> MAVSV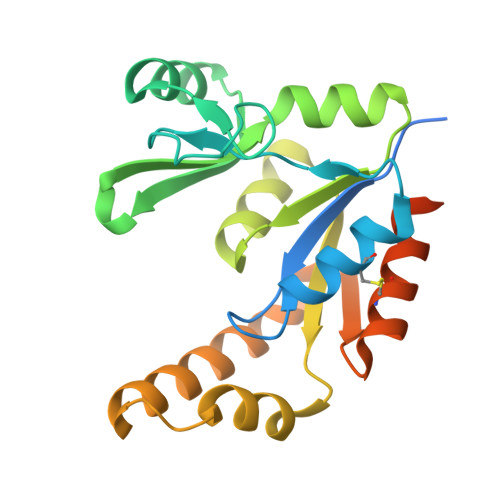GEGPDTKPTARGQPAAVGRVVVLSGPSAVGKSTVVRCLRERIPNLHFSVSATTRCPRPGEVDGVDYHFIDPTRFQQLIDQGELLEWAEIHGGLHRSGTLAQPVRAAAATGVPVLIEVDLAGARAIKKTMPEAVTVFLAPPSWQDLQARLIGRGCETADVIQRRLDTARIELAAQGDFDKVVVNRRLESACAELVSLLVGTAPGSPGVPRGKLAAALEHHHHHH>GHMDLKTAVFNAARDGKLRLLTKLLASKSKEEVSSLISEKTNGATPLLMAARYGHLDMVEFLLEQCSASIEVGGSVNFDGETIEGAPPLWAASAAGHLKVVQSLLNHGASVNNTTLTNSTPLRAACFDGHLEIVKYLVEHKADLEVSNRHGHTCLMISCYKGHKEIAQYLLEKGADVNRKSVKGNTALHDCAESGSLDIMKMLLMYCAKMEKDGYGMTPLLSASVTGHTNIVDFLTHHAQTSKTERINALELLGATFVDKKRDLLGALKYWKKAMNMRYSDRTNIISKPVPQTLIMAYDYAKEVNSAEELEGLIADPDEMRMQALLIRERILGPSHPDTSYYIRYRGAVYADSGNFKRCINLWKYALDMQQSNLDPLSPMTASS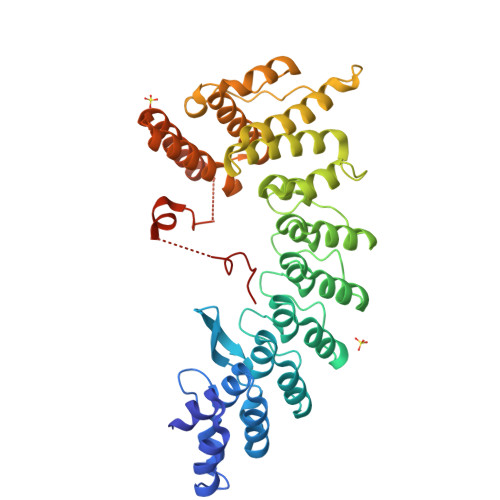LLSFAELFGGGSGGGSGGGSGGGSKKRLLLGLDR[2x]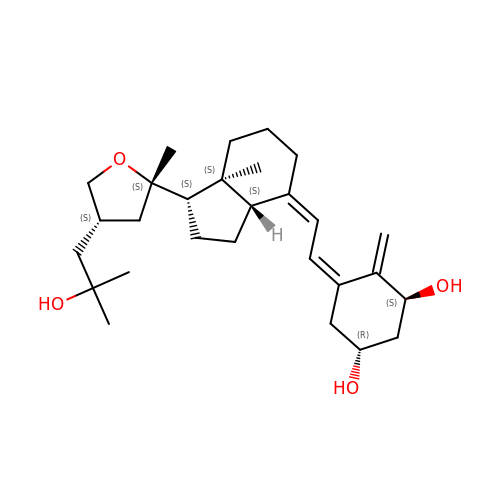(1S,3R,5Z,7E,14beta,17alpha)-17-[(2S,4S)-4-(2-hydroxy-2-methylpropyl)-2-methyltetrahydrofuran-2-yl]-9,10-secoandrosta-5,7,10-triene-1,3-diol | C28 H44 O4 | QFEREDUWILIRPI-VCQGKADLSA-N>MVKVGYIQMEPKILELDKNYSKAEKLIKEASKEGAKLVVLPELFDTGYNFESREEVFDVAQQIPEGETTTFLMELARELGLYIVAGTAEKSGNYLYNSAVVVGPRGYIGKYRKIHLFYREKVFFEPGDL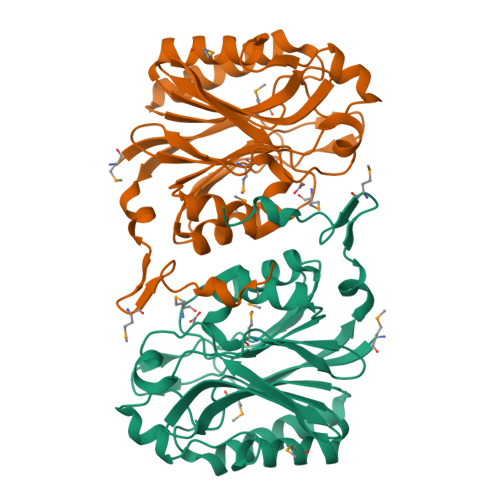GFKVFDIGFAKVGVMICFDWFFPESARTLALKGAEIIAHPANLVMPYAPRAMPIRALENRVYTITADRVGEERGLKFIGKSLIASPKAEVLSIASETEEEIGVVEIDLNLARNKRLNDMNDIFKDRREEYYFR[4x]>[6x]MAFELPNLPYGFRALEPHIDQQTMEIHHDKHHNTYVTKLNAAVEGTDLESKSIEEIVANLDSVPENIQTAVRFNGGGHLNHSLFWELLTPNSEEKGTV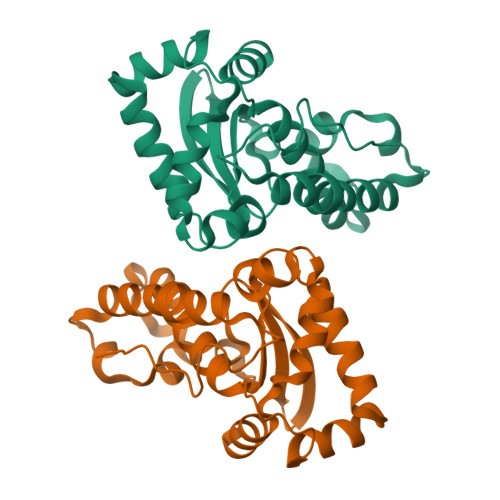VDKIKEQWGSLDAFKEEFANQAAARFGSGWAWLVVNDGKLEIVTTPNQDNPLTEGKTPILGLDVWEHAYYLKYQNKRPDYISAFWNVVNWEKVDELYNAAKHHHHHH> 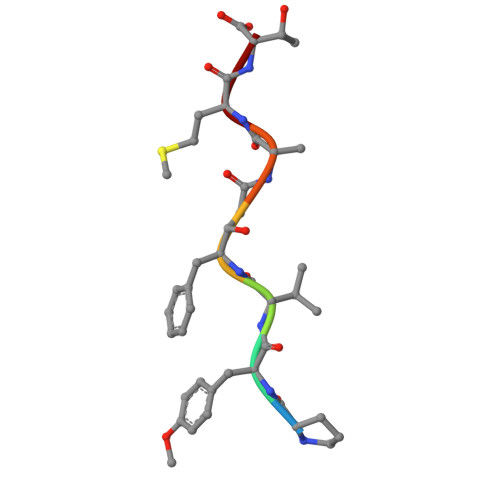PYVFAMT> MEYIIKNGFVYCPLNGVDGEKMDICVKDGKIVESVSDSAKVIDASGKIVMPGGVDPHSHIAGAKVNVGRMYRPEDSKRDAEKFKGGRAGSGFSVPSTFMTGYRYAQMGYTTAMEAAMPPLLARHTHEEFHDTPIIDHAAYPLFGNNWFVMEYLKEGDVDACAAYASWLLRATKGYTIKIVNPAGTEAWGWGGNVHGIYDPAPYFDITPAEIIKGLAEVNEKLQLPHSIHLHCNDLGHPGNYETTLASFDVPKNIKPNPATGSRDTVLYATHVQFHSYGGTTWRDFVSEAPKIADYVNKNDHIVIDVGQITLDETTTMTADGPMEYDLHSLNGLKWANCDVELETGSGVVPFIYSARAPVPAVQWAIGMELFLLIDNPEKVCLTTDSPNAGPFTRYPRVIAWLMSNKYRMNLIEGELHKWAQRKSTVATIDREYTFSEIAQITRATSAKVLGLSDTKGHLGVGADADIAVYDINPETVDPSAEYMAIEEAFSRAACVLKDGEIVVKDGEVVASPHGRTYWVDTQVDESIYSEVLANVESKFKQYYSVNFANYPVQDDYLPKSAP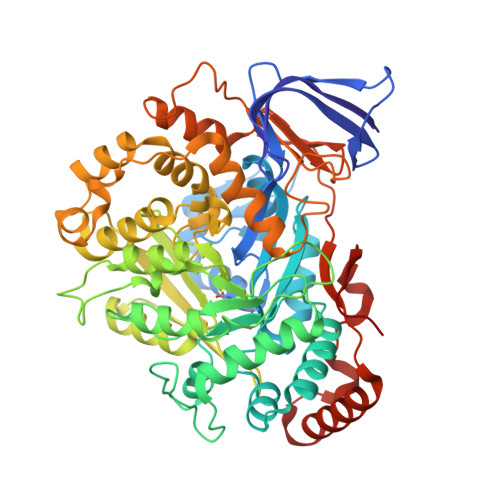VKGVML>MKRRFTLLGSVVALALSSTALASDAPASRGCADDAGWNDPAMPLKVYGNTWYVGTCGISALLVTSDAGHILVDAATPQAGPQILANIRALGFRPEDVRAIVFSHEHFD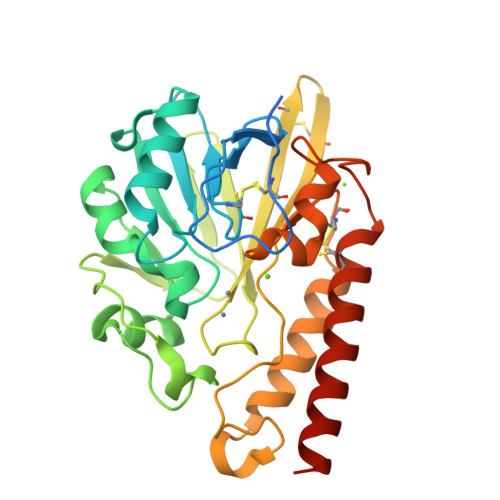HAGSLAELQKATGAPVYARAPAIDTLKRGLPDRTDPQFEVAEPVAPVANIVTLADDGVVSVGPLALTAVASPGHTPGGTSWTWRSCEGDDCRQMVYADSLTAISDDVFRYSDDAAHPGYLAAFRNTLARVAALDCDILVTPHPSASGLWNRIGPRAAAPLMDTTACRRYAQGARQRLEKRLAEEAATSPSSGARP[3x]~{N}2-(1,3-benzodioxol-5-yl)benzene-1,2-diamine 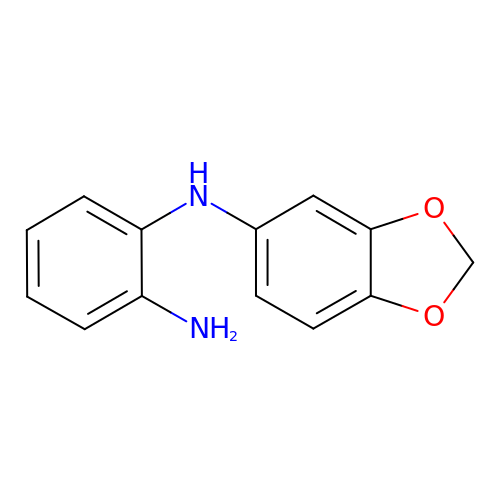| C13 H12 N2 O2 | QMKMDIGODMXIIE-UHFFFAOYSA-N> FSEQTIPPSAKYGGRHTVTMIPGDGIGPELMLHVKSVFRHACVPVDFEEVHVSSNADEEDIRNAIMAIRRNRVALKGNIETNHNLPPSHKSRNNILRTSLDLYANVIHCKSLPGVVTRHKDIDILIVRENTEGEYSSLEHESVAGVVESLAIITKAKSLRIAEYAFKLAQESGRKKVTAVHKANIMKLGDGLFLQCCREVAARYPQITFENMIVDNTTMQLVSRPQQFDVMVMPNLYGNIVNNVCAGLVGGPGLVAGANYGHVYAVFETATRNTGKSIANKNIANPTATLLASCMMLDHLKLHSYATSIRKAVLASMDNENMHTPDIGGQGTTSEAIQDVIRH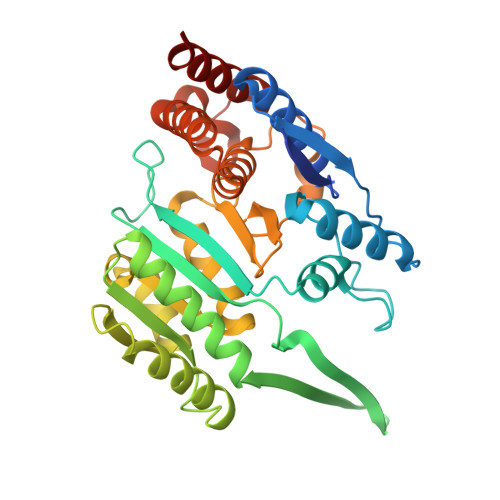IRVINGRAVEA>ASVSAGNSRLLGFDSIPAATTDTISLPKGYKSSVLISWGQPLHKNGPAFDPSGNGTAAAQEVQFGDNNDGMSLFEFPGEKNRALMAINNEYTNYRYLYPHGGMPQSAEDVRKALACEGVSVIEVQRKNGQWQFVQGSRYNRRIHGNSPLRISGPAAGHELMKTSADKHGKKVLGTFQNCANGKTPWGTYLTCEENFTDCFGSSNAQQQFDPAQKRYGVSAASREINWHPFDPRFDMAKNPNELNRHGWVVEIDPFDPQSTPVKRTALGRFKHENAALAETDDG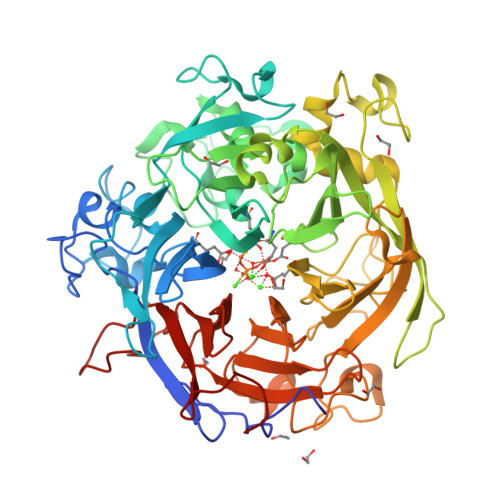RAVVYMGDDERGEFIYKFVSRDKINHRNAKANRDILDHGTLYVARFDAGDGNPDHPKGQGQWIELTHGKNGIDASSGFADQAEVLIHARLAASVVGATRMDRPEWIVVSPKDGQVYCTLTNNAKRGEDGQPVGGPNPREKNVYGQILRWRTDRDDHASKTFAWDLFVVAGNPSVHAGTPKGGSSNITPQNMFNSPDGLGFDKAGRLWILTDGDSSNAGDFAGMGNNQMLCADPATGEIRRFMVGPIGCEVTGISFSPDQKTLFVGIQHPGENGGSTFPEHLPNGKPRSSVMAITREDGGIVGAHHHHHH[2x]>HMSGPRPVVLSGPSGAGKSTLLKRLLQEHSGIFGFSVPHTTRNPRPGEENGKDYYFVTREVMQRDIAAGDFIEHAEFSGNLYGTSKVAVQAVQAMNRICVLDVDLQGVRNIKATDLRPIYISVQPPSLHVLEQRLRQRNTETEESLVKRL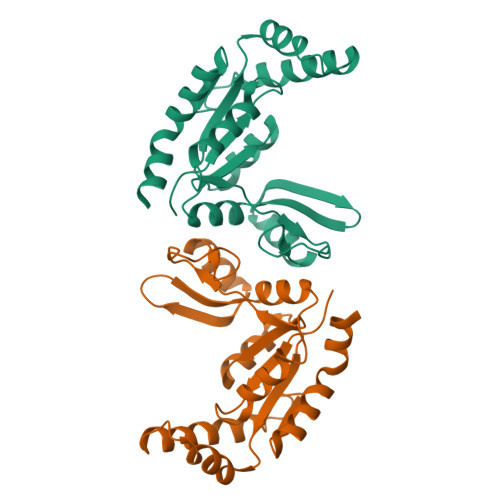AAAQADMESSKEPGLFDVVIINDSLDQAYAELKEALSEEIKKAQRTGA[4x]> MAAPAAEAPLSHVQQALAELAKPKDDPTRKHVCVQVAPAVRVAIAETLGLAPGATTPKQLAEGLRRLGFDEVFDTLFGADLTIMEEGSALLHRLTEHLEAHPHSDEPLPMFTSCCPGWIAMLEKSYPDLIPYVSSCKSPQMMLAAMVKSYLAEKKGIAPKDMVMVSIMPCTRKQSEADRDWFCVDADPTLRQLDHVITTVELGNIFKERGINLAELPEGEWDNPMGVGSGAGVLFGTTGGVMEAALRTAYELFTGTPLPRLSLSEVRGMDGIKETNITMVPAPGSKFEELLKHRAAARAEAAAHGTPGPLAWDGGAGFTSEDGRG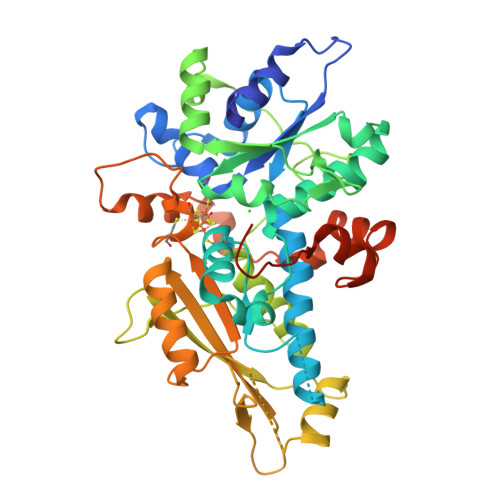GITLRVAVANGLGNAKKLITKMQAGEAKYDFVEIMACPAGCVGGGGQPRSTDKAITQKRQAALYNLDEKSTLRRSHENPSIRELYDTYLGEPLGHKAHELLHTHYVAGGVEEKDEKKSAWSHPQFEK> MRGSHHHHHHTDPATMPFTIDSARGIFPNTLAADVVPATIARFSQLNAEDQLALIWFAYLEMGKTLTIAAPGAASMQLAENALKEIQAMGPLQQTQAMCDLANRADTPLCRTYASWSPNIKLGFWYRLGELMEQGFVAPIPAGYQLSAN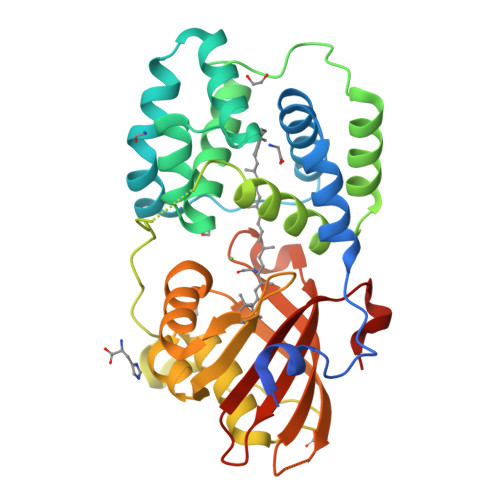ANAVLATIQGLESGQQITVLRNAVVDMGFTAGKDGKRIAEPVVPPQDTASRTKVSIEGVTNATVLNWMDNLNANDFDTLIELFTSDGALQPPFQRPIVGKENVLRFFREECQNLKLIPERGVTEPAEDGFTQIKVTGKVQTPWFGGNVGMNIAWRFLLNPEGKIFFVAIDLLASPKELLNFAR>MFNQFNPLVYTHGGKLERKSKKDKTASKVFEEFGVMEAYNCWKEASLCIQQRDKDSVLKLVAALNTYKDAVEPIFDSRLNSAQEVLQPSILEEFFEYLFSRIDSIVGVNIPIRHPAKGYLSLSFNPHNIETLIQSPEYTVRAKDHDFIIGGSAKLTIQGHGGEGETTNIVVPAVAIECKRYLERNMLDECAGTAERLKRATPYCLYFVVAEYLKLDDGAPELTEIDEIYILRHQRNSERNKPGFKPNPIDG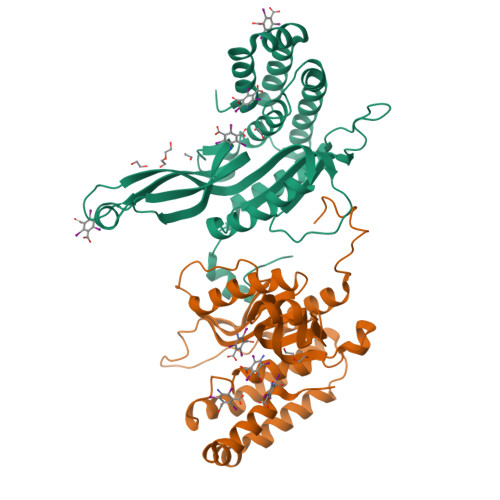ELIWDLYQEVMNHLGKIWWDPNSALQRGKVFNRP[2x]The third enzyme is 2-C-Methyl-d-erythritol-4-phosphate cytidyltransferase (IspD), 4-diphosphocytidyl-2-C-methyl-d-erythritol (CDPME) is formed from MEP by reaction with CTP12. The subunit structure of BsIspD was of a compact α/β fold from which a long β-meander extended. The core of the enzyme consisted of a seven β-sheets (β2, β1, β4, β9, β5, β8, β10) where all strands were parallel, apart from β8 and β2. The β-meander lay between antiparallel strands β6 and β7 and made the major contribution to the dimer interface, and the lesser contribution came from the side-chain interactions of the residues on the α-helix fragment at the C-terminus.

Furthermore, the structure of BsIspD/CTP-Mg2+ complex was determined, the final model revealed two molecules in one asymmetric unit, named molecule D and E, respectively. These two subunits can be superimposed with a r.m.s.d of 0.63 Å for 215 Cα. Moreover, the average B factor of the main-chain and side-chain of the molecule D was about 20 Å lower than that in the molecule E, which implied that molecule D was in more stable state than molecule E. Six residues (227–232) in the C-terminal of two molecules were missed in the final model. In addition, the ribose was hydrogen bonded to Pro8, Gly11, Gly105 and Ala106 (Gly11 N-ribose O2′ = 3.0 Å; Pro8 O-ribose O3′ = 2.9 Å, Gly105 N-ribose O3′ = 3.3 Å and Ala106 N-ribose O3′ = 3.3 Å). The triphosphate wrapped around a magnesium ion, coordination bonds were formed between the magnesium ion and the oxygen atoms of α-, β-, γ-phosphate in CTP. In the BsIspD/CTP-Mg2+ complex, it was clearly seen that the P-loop had shifted away from the active site upon CTP binding, and it changed from beta-alpha (β-α) form to alpha-beta (α-β) form32. The Cα atoms of Gly11,Gln12 and Arg15 shifted 4.4 Å, 7.6 Å and 7.9 Å, respectively, in this way, the P-loop did not interact with residues Asp84, Asp104, Ala106, and Lys 209 anymore, the active pocket was open to accommodate CTP, the P-loop and the residues Lys209 and Ala106 were involved in the interactions with CTP. The L1-loop rotated about 30° and moved about 2.4 Å, a cleft in 4 Å width was formed between the L1-loop and P-loop, favoring for the binding of the cytosine base of CTP. Meanwhile, it was observed the L2-loop shifted about 2 Å, the residue Thr211 was hydrogen bonded to the residue Arg15 in the P-loop (3.5 Å).

>MSYDVVIPAAGQGKRMKAGRNKLFIELKGDPVIIHTLRVFDSHRQCDKIILVINEQEREHFQQLLSDYPFQTSIELVAGGDERQHSVYKGLKAVKQEKIVLVHDGARPFIKHEQIDELIAEAEQTGAAILAVPVKDTIKRVQDLQVSETIERSSLWAVQTPQAFRLSLLMKAHAEAERKGFLGTDDASLVEQMEGGSVRVVEGSYTNIKLTTPDDLTSAEAIMESESGNKHV[2x]> GLPTELKPGTNQFLTTDDGTSPPILPGFEPTPLIHIPGEFTSLLDLCRIETILEVNNTTGTTGVNRLLIPVRAQNNVDQLCASFQVDPGRNGPWQSTMVGQICRYYTQWSGSLKVTFMFTGSFMATGKMLIAYTPPGSAQPTTREAAMLGTHIVWDFGLQSSVTLVIPWISNTHFRAVKTGGVYDYY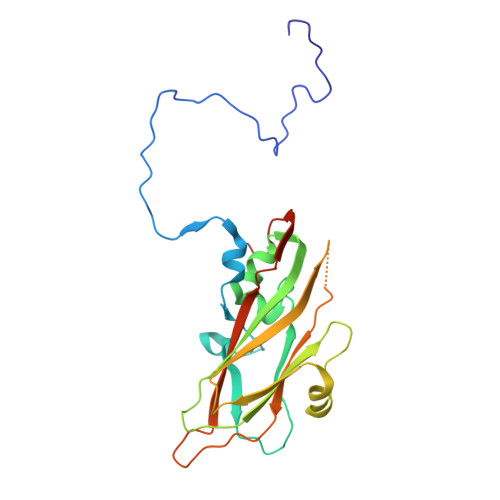ATGIVTIWYQTNFVVPPDTPSEANIIALGAAQENFTLKLCKDTDEIRQTAEYQN> GQEEPSKVALSYSKSLKAPETDSLNLPVDENGYITIFDGETFNGWRGYGKDRVPTKWTIEDGCIKFNGSGGGEAQDGDGGDLIFAHKFKNFELELEWKVAKGSNSGILYLAQEVTSKDKDGNDVLEPIYISAPEYQILDNANHPDAKLGKDNNRQSASLYDMIPAV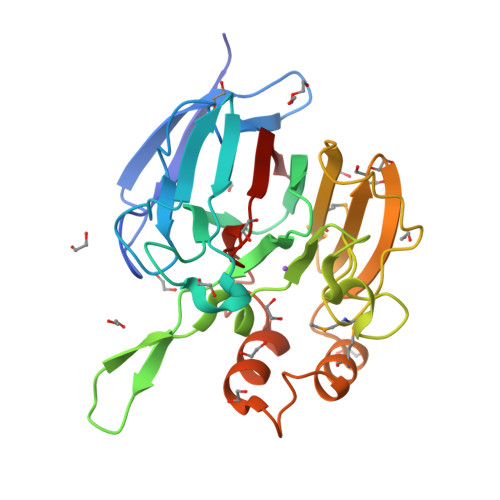PQNSKPFGEWNKAKIMVYKGTVVHGQNDENVLEYHLWTKQWTDMLQASKFSEDKWPLAFELLNNCGGENHEGFIGLQDHGDDVWFRNIRVKVLD> MVSSDRPVSLEDEVSHSMKEMIGGCCVCSDERGWAENPLVYCDGHGCSVAVHQACYGIVQVPTGPWFCRKCESQERAARVRCELCPHKDGALKRTDNGGWAHVVCALYIPEVQFANVSTMEPI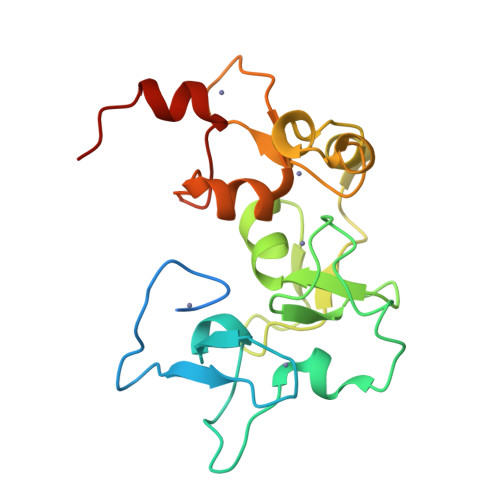VLQSVPHDRYNKTCYICDEQGRESKAATGACMTCNKHGCRQAFHVTCAQFAGLLCEEEGNGADNVQYCGYCKYHFSKLKKSKRGS> ESNDSGIVVYNAQHENLVKSWVDGFTKDTGIKVTLRNGGDSELGNQLVQEGSASPADVFLTENSPAMVLVDNAKLFAPLDAVTQAQVAQEYRPEHGRWTGIAARSTVFVYNPEKISEAELPKSIMDLAKP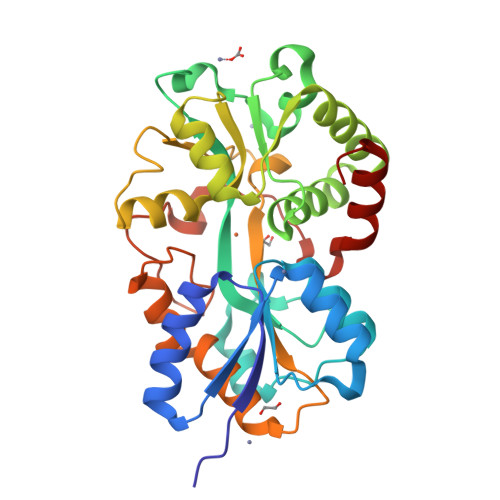EWKGRWAASPSGADFQAIVSAMLELKGEKATLEWLKAMKTNFTAYKGNSTVMKAVNAGQIDGGVIYHYYRFVDQAKTGENSGKTQLHYFKHQDPGAFVSISGGGVLASSKHPKEAQEFVKWITGKSGQDILRTNNAFEYAVGVDAASNPKLVPLKDLDAPKVEPSKLNSKKVVELMTEAGLL> 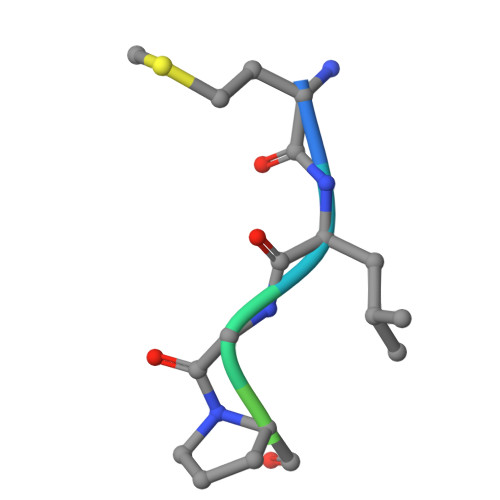MLGPEGGRWG>MNTNKATATYLKSIMLPETGPASIPDDITERHILKQETSSYNLEVSESGSGILVCFPGAPGSRIGAHYRWNANQTGLEFDQWLETSQDLKKAFNYGRLISRKYDIQSSTLPAGLYALNGTLNAATFEGSLSEVESLTYNSLMSLTTNPQDKVNNQLVTKGVTVLNLPTGFDKPYVRLEDETPQGLQSMNGAKMRCTAAIAPRRYEIDLPSQRLPPVPATGTLTTLYEGNADIVNSTTVTGDINFGLARQPADETTFHFQLDFMGLDNDVPVVTVVSSALATTDNHRGVSAKMTQSIPTENITKPITRVKLSYKINQQTAIDNVATLGTMGPASVSFSSGNGNVPGVLRPITLVAYEKMTPLSILTVAGVSNYELIPNPELLKNMVTRYGKYDPEGLNYAKMILSHREELDIRTVWRTEEYKERTRVFNEITDFSSDLPTSKAWGWRDIVRGIRKVAAPVLSTLFPMAAPLIGMADQFIGDLTKTNAAGGRYHSMAAGGRYKDVLESWA[13x]

The infectious pancreatic necrosis virus (IPNV), a member of the Aquabirnavirus, can infect diverse salmonid species, leading to lethal outcomes characterized by pancreatic necrosis and catarrhal enteritis. Birnaviruses have a bi-segmented dsRNA genome. On the contrary, VP2s assemble into a 60–70 nm T=13 icosahedral single-layer capsid to protect the RNPs. The VP2 subunits are organized into three domains: the α-helix-rich N and C-terminal base (B) domain located on the capsid interior; the conserved β-barrel jelly roll fold shell (S) domain; and the unique β-barrel jelly roll fold projection (P) domain, which is situated on the capsid exterior.

The first infectious IPNV capsid structure was determined at a resolution of 2.75 Å using cryo-EM single particle analysis with imposed icosahedral symmetry. From another perspective, five subunits (a) form a pentagonal unit at the 5-fold axis, while the remaining subunits contribute to hexagonal units in the capsid. While the overall structure of the VP2 subunits is similar, notable structural variations are observed in the C-terminal region of the B domain (residues 429–435) and the variable loop region of the S domain (residues 110–117) (5-fold, down, and up conformations). A comparison between the cryo-EM structures of the infectious T=13 IBDV and IPNV particles similarly reveals differences in these surface loops, reinforcing earlier observations made from the T=1 structures. Both IPNV and IBDV form four corresponding surface loops: L1 (IPNV: 206–222, IBDV: 204–222), L2 (IPNV: 245–260, IBDV: 245–260), L3 (IPNV: 277–287, IBDV: 277–284), and L4 (IPNV: 313–323, IBDV: 313–322), while an additional loop, L4′ (326-334), is unique to IPNV. However, the variable loop of the other 12 VP2 subunits in the asymmetric unit adopts either an up or down conformation, contributing to the formation of the necessary structural interfaces within the hexagonal capsomers in the T=13 capsid lattice. The Tyr115 residues of the three up conformations largely contribute to forming the interface. Specifically, this intensity was observed from Glu429 to Ser435 in subunit (a), Glu429 to Ile430 in subunit (b), and Glu429 to Ser434 in subunit (c). The C-terminal extensions create an additional hydrophobic interface and interlock with neighboring subunits on the capsid interior.(2E)-2-[({3-hydroxy-2-methyl-5-[(phosphonooxy)methyl]pyridin-4-yl}methyl)amino]-4-(methylsulfanyl)but-2-enoic 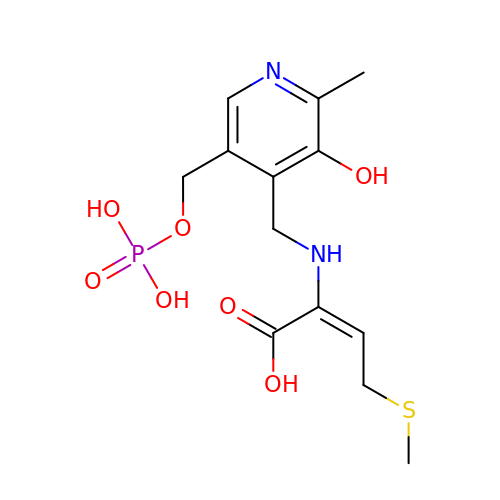acid | C13 H19 N2 O7 P S | LPFNPHQQDYAHKU-QDEBKDIKSA-N> XMEAAHSKSTEECLAYFGVSETTGLTPDQVKRHLEKYGHNELPAEEGKSLWELVIEQFEDLLVRILLLAACISFVLAWFEEGEETITAFVEPFVILLILIANAIVGVWQERNAENAIEALKEYEPEMGKVYRADRKSVQRIKARDIVPGDIVEVAVGDKVPADIRILSIKSTTLRVDQSILTGESVSVIKHTEPVPDPRAVNQDKKNMLFSGTNIAAGKALGIVATTGVSTEIGKIRDQMAATEQDKTPLQQKLDEFGEQLSKVISLICVAVWLINIGHFNDPVHGGSWIRGAIYYFKIAVALAVAAIPEGLPAVITTCLALGTRRMAKKNAIVRSLPSVETLGCTSVICSDKTGTLTTNQMSVCKMFIIDKVDGDFCSLNEFSITGSTYAPE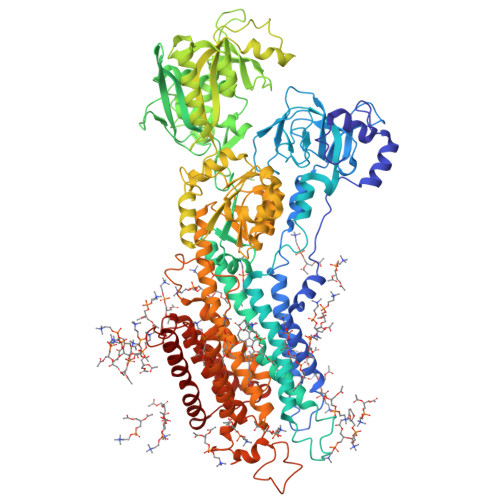GEVLKNDKPIRSGQFDGLVELATICALCNDSSLDFNETKGVYEKVGEATETALTTLVEKMNVFNTEVRNLSKVERANACNSVIRQLMKKEFTLEFSRDRKSMSVYCSPAKSSRAAVGNKMFVKGAPEGVIDRCNYVRVGTTRVPMTGPVKEKILSVIKEWGTGRDTLRCLALATRDTPPKREEMVLDDSSRFMEYETDLTFVGVVGMLDPPRKEVMGSIQLCRDAGIRVIMITGDNKGTAIAICRRIGIFGENEEVADRAYTGREFDDLPLAEQREACRRACCFARVEPSHKSKIVEYLQSYDEITAMTGDGVNDAPALKKAEIGIAMGSGTAVAKTASEMVLADDNFSTIVAAVEEGRAIYNNMKQFIRYLISSNVGEVVCIFLTAALGLPEALIPVQLLWVNLVTDGLPATALGFNPPDLDIMDRPPRSPKEPLISGWLFFRYMAIGGYVGAATVGAAAWWFMYAEDGPGVTYHQLTHFMQCTEDHPHFEGLDCEIFEAPEPMTMALSVLVTIEMCNALNSLSENQSLMRMPPWVNIWLLGSICLSMSLHFLILYVDPLPMIFKLKALDLTQWLMVLKISLPVIGLDEILKFIARNYLEG> PSKFSKEQLRTFQMIHENFGRALSTYLSGR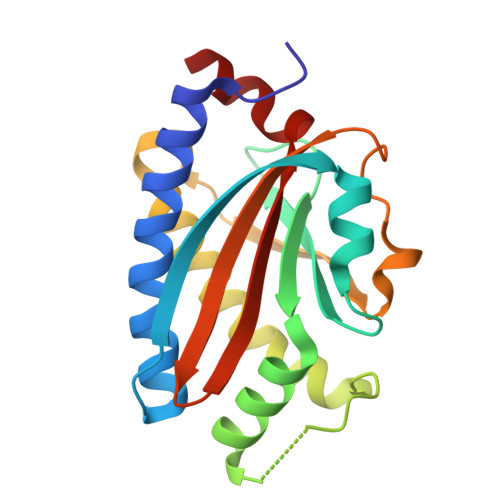LRTFVDVEISIDQLTYEEFIRSVMIPSFIVIFTGDVFEGSAIFEMRLDLFYTMLDIIMGGPGENPPNRPPTEIETSIMRKEVTNMLTLLAQAWSDFQYFIPSIENVETNPQFVQIVPPNEIVLLVTASVSWGEFTSFINVCWPFSLLEPLLEK>[2x]GSMISTLEDVLSLLDLQQIDDAAFVGTQPDTPNHHIIGSQVAAQALMAAGRTTP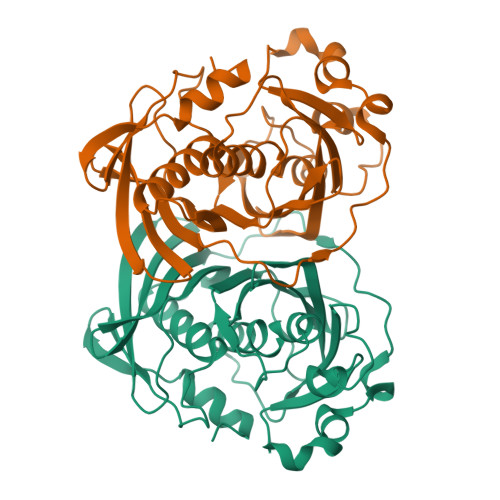GRLAHSMHMYFLRRGDARQPIQYDVTPLRDGGTISSRRVTASQSGVVLFEALASFTIIADDVDWQQRMPDVAGPSAVHGLEDLLAPYAEEFGDWWPQQRPFTMRYLDAPPRVALDLSDPPPPRLRIWLRANGEVTDDPLVNSCVVAYLSALTLLECVMTTMRTTPVGPRLSALVDHTIWFHRAADFTDWLLFDQFSPSIVGRRGLATGTLYNRSGELVCIATQEGYFAEQRQ> LLEAIAIALTAAHFGAPLLYYWRAKRWLKKPWDVAPDPTYRPRVTVIVPTYNEAPLIEEKLDNIYEQDYPRDKLEVVVVDSASTDGTPSA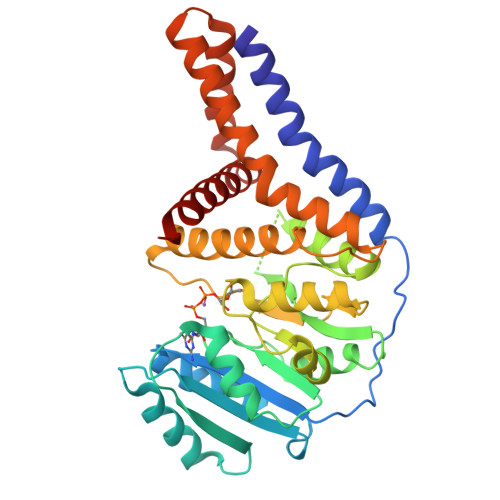VRRWAETHPDLALTLVEETERRGKAHALNTALRHATGEIVVITDADALWPARDTLANAVKWLADPTVGAVSCVKRPAGPAGVEDSYRDFYNVLRVAESKAWATPIFHGELAAFKRELLERLGGFPTDVGADDSHTATKIAMMGYRAITPPDVVCVEAVPKRGYHAWRIRRAQHLVQHFAKAIRDGKAPPPFKPILHAEAYLHLANPWALPTAAAALAAAAAAGSLPAAALLATGAALALYKPYRTWTTMQAYLIAAAVKNLWDKE;> MLLEAIAIALTAAHFGAPLLYYWRAKRWLKKPWDVAPDPTYRPRVTVIVPTYNEAPLIEEKLDNIYEQDYPRDKLEVVVVDSASTDGTPSAVRRWAETHPDLALTLVEETERRGKAHALNTALRHATGEIVVITDADALWPARDTLANAVKWLADPTVGAVSCVKRPAGPAGVEDSYRDFYNVLRVAESKAWATPIFHGELAAFKRELLERLGGFPTDVGADDSHTATKIAMMGYRAITPPDVVCVEAVPKRGYHAWRIRRAQHLVQHFAKAIRDGKAPPPFKPILHAEAYLHLANPWALPTAAAALAAAAAAGSLPAAALLATGAALALYKPYRTWTTMQAYLIAAAVKNLWDKE> LEERATGGYVQNPSGSASFTMYSGCGSPACGETASGYTAAMNQLSFGAGPGAGAGDACGRCFALTGTADPYSPSYTGPFHTIVVKVTDLCPVAGNQEWCGQTTSNPNNQHGEPVHFDICEDTGGAGAFFPSGHGALTGTYREVSCSQWSGSDGSPLWTGACLSGESAANWPSTACGNKGTAPS

Here we describe the first crystal structure of a beta‐1,4‐endoglucanase from a brown‐rot fungus, Gloeophyllum trabeum GtCel45A, which belongs to subfamily C of glycoside hydrolase family 45 (GH45). The enzyme consists of a single catalytic module folded into a six‐stranded double‐psi beta‐barrel domain surrounded by long loops. GtCel45A is very similar in sequence (82% identity) and structure to PcCel45A from the white‐rot fungus Phanerochaete chrysosporium.

GtCel45A is ~ 18 kDa in size and the crystal structure contains 179 amino acids. The structure is refined at 1.30 Å resolution and R free 0.18. Surprisingly though, initial hydrolysis of barley beta‐glucan was almost twice as fast in GtCel45A as compared to PcCel45A.alpha-D-glucopyranosyl fluoride 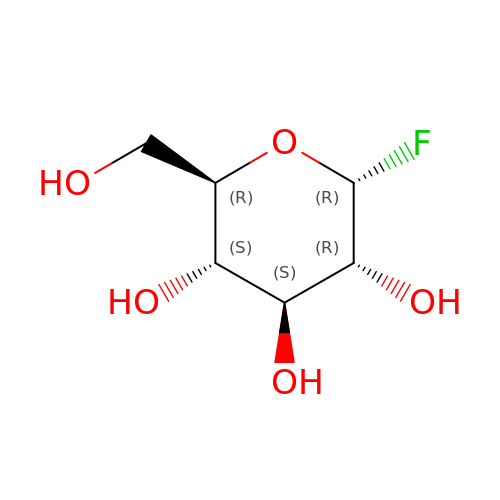| C6 H11 F O5 | ATMYEINZLWEOQU-DVKNGEFBSA-N>[3x]XEWEALEKKCAALE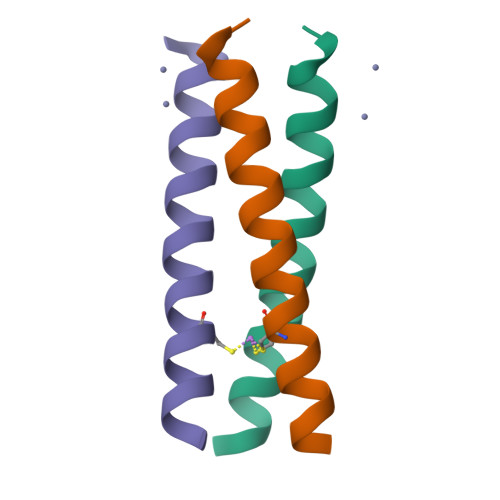SKLQALEKKLEALEHGX>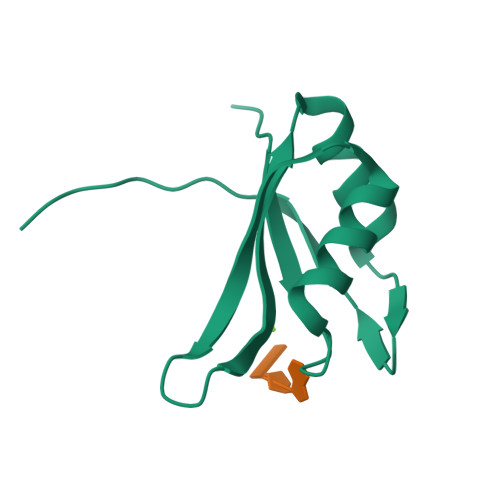 GPSRVVYLGSIPYDQTEEQILDLCSNVGPVINLKMMFDPQTGRSKGYAFIEFRDLESSASAVRNLNGYQLGSRFLKCGYSSNSDISGVSQQQQQQYN>FQGAMDPEFSMKIGIIGAMEEQVTLLRDKIENRQTISLGGCEIYTGQLNGTEVALLKSGIGKVAAALGATLLLEHCKPDVIINTGSAGGLAPTLKVGDIVVSDEARYHDADVTAFGYEYGQLPGCPAGFKADDKLIAAAEACIAELNLNAVRGLIVSGDAFI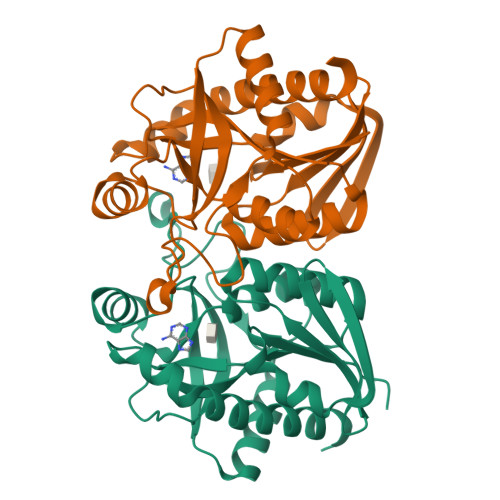NGSVGLAKIRHNFPQAIAVEMEATAIAHVCHNFNVPFVVVRAISDVADQQSHLSFDEFLAVAAKQSSLMVESLVQKLAHG[2x]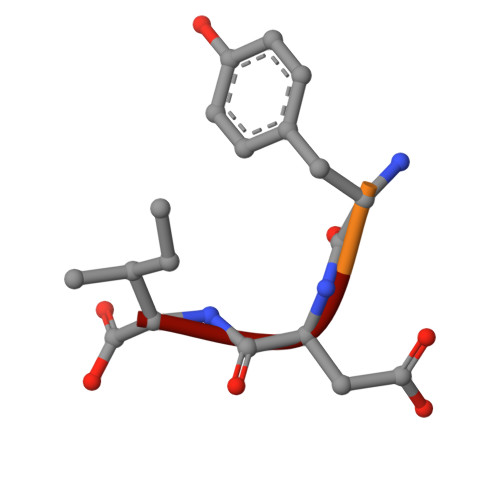> MNYDI>GRPYKLLNGIKLGVYIPQEWHDRLMEIAKEKNLTLSDV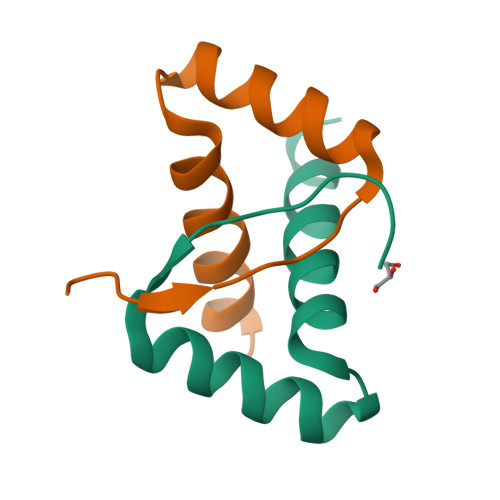CRLAIKEYLDNHDKQKK[2x]>GPHMPGSGQIQLWQFLLELLSDSANASCITWEGTNGEFKMTDPDEVARRWGERKSKPNMNYDKLSRALRYYYDKNIMTKVHGK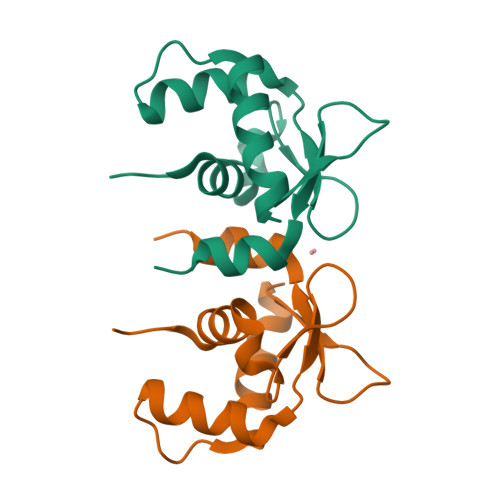RYAYKFDFHGIAQALQPHPTESSMYKYPSDISYMPSYHAHQQKVN[4x]>GAMDPDLEATLRAIVHSATSLVDARYGAMEVHDRQHRVLHFVYEGIDEETVRRIGHLPKGLGVIGLLIEDPKPLRLDDVSAHPASIGFPPYHPPMRTFLGVPVRVRDESFGTLYLTDKTNGQPFSDDDEVLVQALAAAAGI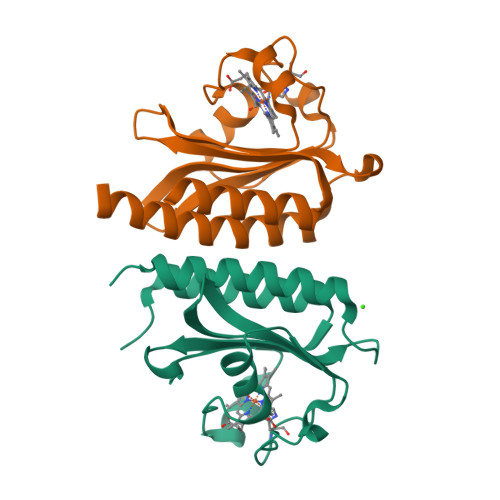AVANARLYQQAK[2x]> MDYKDDDDKGPKREAVQEERQRNKEKSENEVESTSNSQNDMPI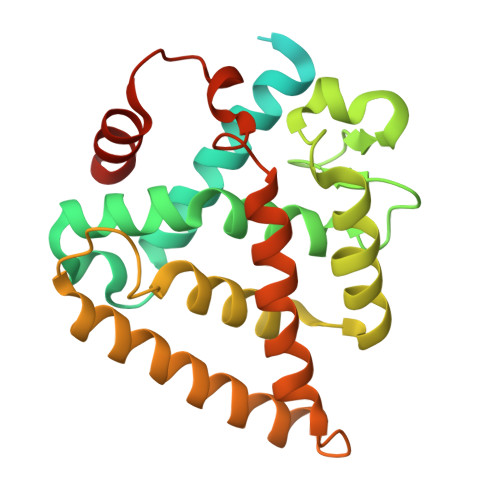ERILEAELRVEPKNEDIDSRDPVSDICQAADRQLYQLIEWAKHIPHFTELPVEDQVILLKSGWNELLIAGFSHRSMSVKDGIMLATGLVVHRNCAHQAGVGAIFDRVLTELVAKMREMKMDKTELGCLRSIVLFNPEAKGLKSTQQVENLREKVYAILEEYCRQTYPDQSGRFAKLLLRLPALRSIGLKCLEHLFFFKLVGNTSIDSFLLSMLESNSDS> SLYKTFFKRNAVFVGTIFAGAFVFQTVFDTAITSWYE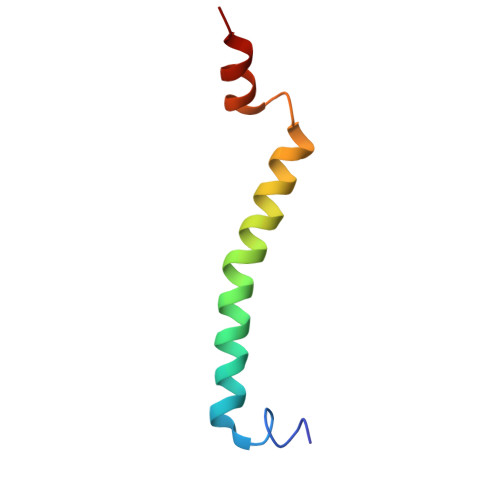NHNKGKLWKDVKARIAA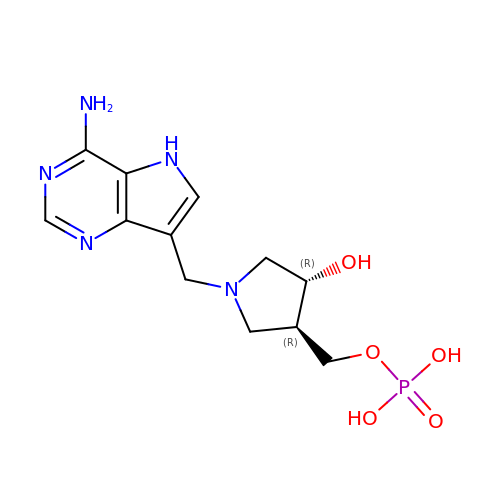{(3R,4R)-1-[(4-amino-5H-pyrrolo[3,2-d]pyrimidin-7-yl)methyl]-4-hydroxypyrrolidin-3-yl}methyl dihydrogen phosphate | C12 H18 N5 O5 P | QPUSNADQSHKIFF-BDAKNGLRSA-N> MTVFRQENVDDYYDTGEELGSGQFAVVKKCREKSTGLQYAAKFIKKRRTKSSRRGVSREDIEREVSILKEIQHPNVITLHEVYENKTDVILILELVAGGELFDFLAEKESLTEEEATEFLKQILNGVYYLHSLQIAHFDLKPENIMLLDRNVPKPRIKIIDFGLAHKIDFGNEFKNIFGTPEFVAPEIVNYEPLGLEADMWSIGVITYILLSGASPFLGDTKQETLANVSAVNYEFEDEYFSNTSALAKDFIRRLLVKDP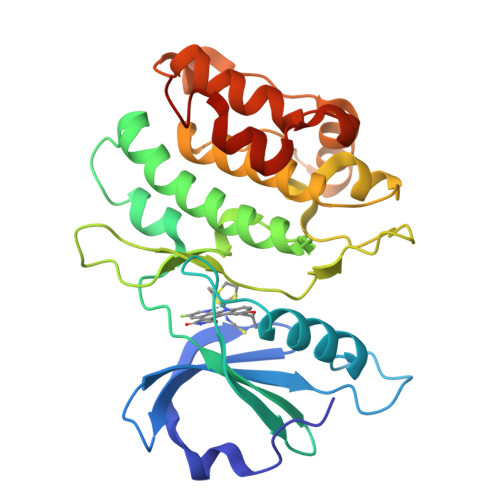KKRMTIQDSLQHPWIKPKDTQQALS>AGLSPEEQIETRQAGYEFMGWNMGKIKANLEGEYNAAQVEAAANVIAAIANSGMGALYGPGTDKNVGDVKTRVKPEFFQNMEDVGKI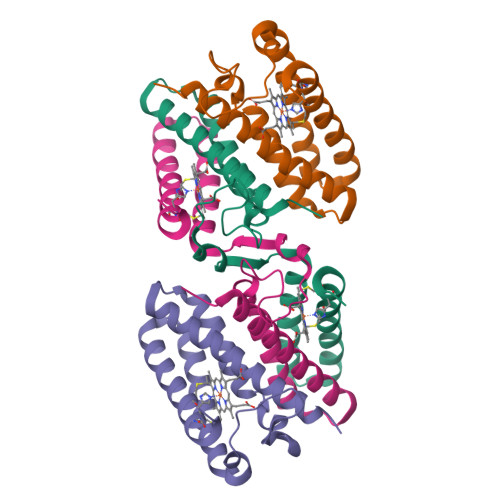AREFVGAANTLAEVAATGEAEAVKTAFGDVGAACKSCHEKYRAK[8x]>MATAQSNSPRVFCIGTADTKFDELRFLSEHVRSSLNSFSNKSSFKVGVTVVDVSTSWKETNSCADFDFVPSKDVLSCHTLGEETMGTFADTRGLAIAIMSKALETFLSIANDEQNLAGVIGLGGSGGTSLLSSAFRSLPIGIPKVIISTVASGQTESYIGTSDLVLFPSVVDICGINNVSKVVLSNAGAAFAGMVIGRLESSKEHSITNGKFTVGVTMFGVTTPCVNAVKERLVKEGYETLVFHATGVGGRAMEDLVRGGFIQGVLDITTTEVADYVVGGVMACDSSRFDAILEKKIPLVLSVGALDMVNFGPKTTIPPEFQQRKIHEHNEQVSLMRTTVGENKKFAAFIAEKLNKASSSVCVCLPEKGVSALDAPGKDFYDPEATSCLTRELQMLLENNERCQVKVLPYHINDAEFANALVDSFLEISPK[2x];>[2x]SYTRSEEIESLEQFHMATASSLIHKQMCSIVYTGPLKVQQMKNFIDSLVASLSAAVSNLVKILKDTAAIDLETRQKFGVLDVASKRWLVKPSAKNHAWGVVETHARKYHVALLEHDEFGIITCDNWRRVAVSSESVVYSDMAKLRTLRRLLKDGEPHVSSAKVVLVDGVPGCGKTKEILSRVNFEEDLILVPGRQAAEMIRRRANASGIIVATKDNVRTVDSFLMNYGKGARCQFKRLFIDEGLMLHTGCVNFLVEMSLCDIAYVYGDTQQIPYINRVTGFPYPAHFAKLEVDEVETRRTTLRCPADVTHFLNQRYEGHVMCTSSEKKSVSQEMVSGAASINPVSKPLKGKILTFTQSDKEALLSRGY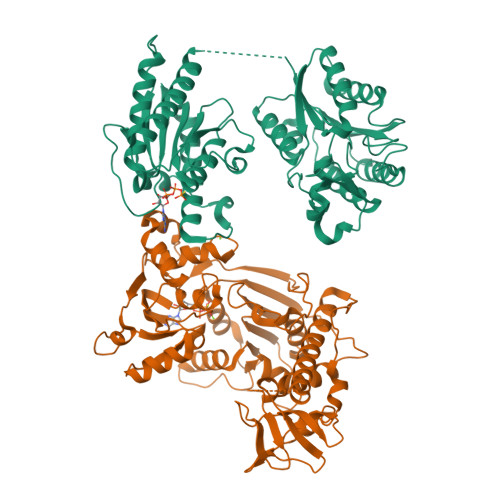ADVHTVHEVQGETYADVSLVRLTPTPVSIIARDSPHVLVSLSRHTKSLKYYTVVMDPLVSIIRDLERVSSYLLDMYKVDAGTQ>[2x]PPSVFAEVPQAQPVLVFKLTADFREDPDPRKVNLGVGAYRTDDCHPWVLPVVKKVEQKIANDNSLNHEYLPILGLAEFRSCASRLALGDDSPALKEKRVGGVQSL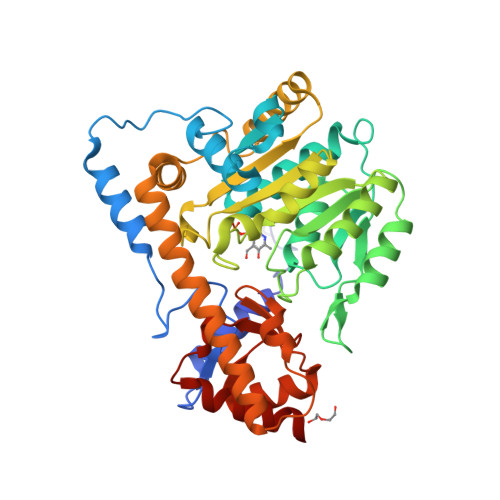GGTGALRIGADFLARWYNGTNNKNTPVYVSSPTWENHNAVFSAAGFKDIRSYRYWDAEKRGLDLQGFLNDLENAPEFSIVVLHACAHNPTGIDPTPEQWKQIASVMKHRFLFPFFDSAYQGFASGNLERDAWAIRYFVSEGFEFFCAQSFSKNFGLYNERVGNLTVVGKEPESILQVLSQMEKIVRITWSNPPAQGARIVASTLSNPELFEEWTGNVKTMADRILTMRSELRARLEALKTPGTWNHITDQIGMFSFTGLNPKQVEYLVNEKHIYLLPSGRINVSGLTTKNLDYVATSIHEAVTKIQ>GFGNQGGFGNSRGGGAGLGNNQGSNMGGGMNFGAFSINPAMMAAAQAALQSSWGMMGMLASQQN[6x];>[6x]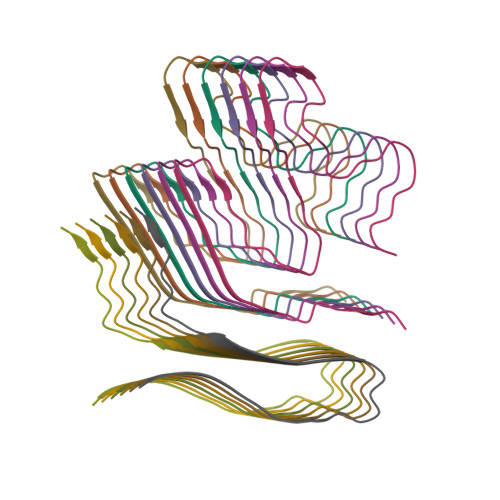LDNVATYAGQFNQDYLSGMAANMSGTFGGANMPNLY Neuronal nicotinic acetylcholine receptors (nAChRs) are a group of ligand-gated cation-selective ion channels that play key roles in fast signal transmission in the nervous system. On the other hand, the crystal structure of the acetylcholine-binding proteins (AChBPs) from mollusks, which are soluble homologs of the extracellular domain (ECD) of nAChR, represented a great leap in the understanding of the structure and function of nAChRs. Interestingly, despite the only 20%–24% sequence identity with nAChRs, AChBPs display a striking structural resemblance to the nAChR ECD, and their pharmacological properties closely resemble those of nAChRs. The α-conotoxins display a consensus fold with a central helical region braced by two conserved disulfide bridges.

To reveal the mechanism responsible for the distinctive binding profile and selectivity of LvIA towards different α3*nAChRs, we solved the crystal structure of α-conotoxin LvIA in complex with the acetylcholine binding protein from Aplysia californica (Ac-AChBP) at 3.4 Å resolution. The protein forms a windmill-like pentamer along a five-fold axis, forming five highly similar ligand-binding sites between two adjacent protomers. Each α-CTx molecule interacts with two adjacent Ac-AChBP protomers at their interface, forming the principal and complementary binding sides. Most interactions on the principal side were between the peptide and the C-loop (Gln-184~Tyr-193) of one of the Ac-AChBP protomers. Upon binding to LvIA, the C-loop has a significant conformational change that was also observed in the complex structures of Ac-AChBP with other α-CTxs. His-5 forms a hydrogen bond with Tyr-91, Pro-6 undergoes a hydrophobic interaction with Tyr-91 and Trp-145, Ala-7 displays extensive hydrophobic interactions with Trp-145, Val-146, Tyr-147, and Tyr-193, while a salt bridge between His-12 of α-CTx LvIA and Glu-191 of Ac-AChBP was also observed. In addition, the Cys-2/Cys-8 disulfide bridge of the peptide was found to be stacked against the vicinal Cys-188/Cys-189 disulfide bond of Ac-AChBP. On the complementary binding side, Ser-4 and Asn-9 of LvIA form hydrogen bonds with Ser-165 and Gln-55 of Ac-AChBP, respectively. An electronic interaction was also observed between Asp-11 of LvIA and Arg-77 of Ac-AChBP. Among the studied mutants, H5A, P6A, and H12A completely lost their binding capacity for Ac-AChBP.

>SQANLMRLKSDLFNRSPMYPGPTKDDPLTVTLGFTLQDIVKVDSSTNEVDLVYYEQQRWKLNSLMWDPNEYGNITDFRTSAADIWTPDITAYSSTRPVQVLSPQIAVVTHDGSVMFIPAQRLSFMCDPTGVDSEEGVTCAVKFGSWVYSGFEIDLKTDTDQVDLSSYYASSKYEILSATQTRQVQHYSCCPEPYIDVNLVVKFRERRAGNGFFRNLFDHHHHHH[5x];>[5x]GCCSHPACNVDHPEICX(10R,13S)-16-amino-13-hydroxy-7,13-dioxo-8,12,14-trioxa-13lambda~5~-phosphahexadecan-10-yl hexadecanoate | C28 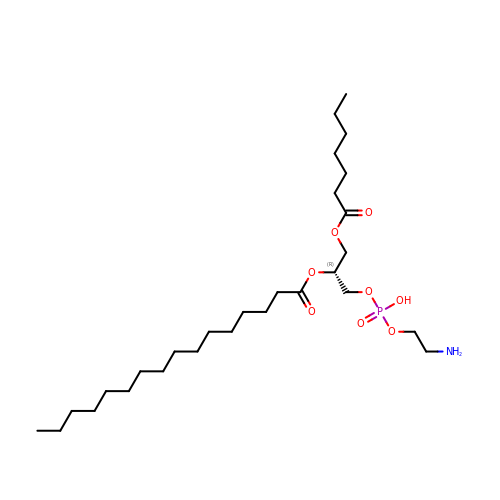H56 N O8 P | AALSRRWRFFTHRD-AREMUKBSSA-N[[(2~{R},3~{R},4~{S},5~{R})-5-[2-chloranyl-6-[(phenylmethyl)amino]purin-9-yl]-4-fluoranyl-3-oxidanyl-oxolan-2-yl]methoxy-oxidanyl-phosphoryl]methylphosphonic acid | C18 H21 Cl F N5 O8 P2 | 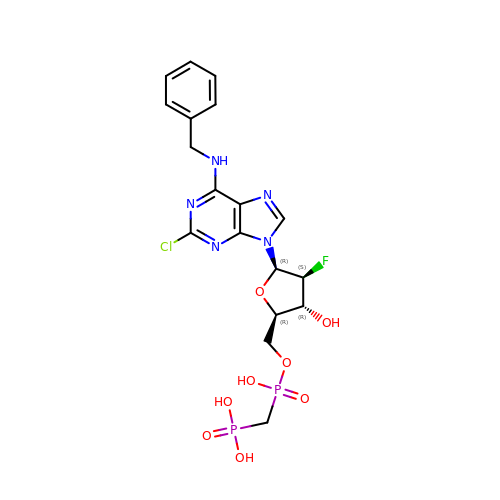PPWDVNAHTXSWKW-DMVWFOPNSA-N propane-1,2,3-triyl 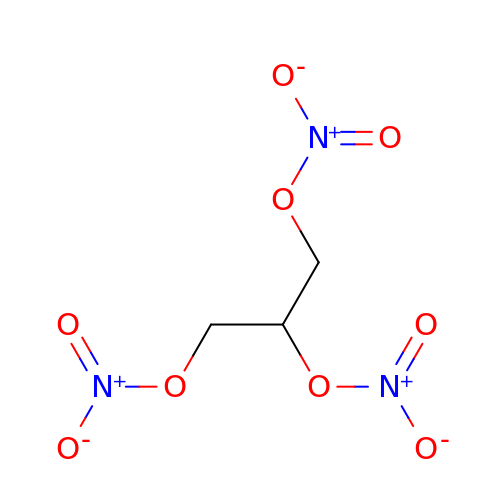trinitrate | C3 H5 N3 O9 | SNIOPGDIGTZGOP-UHFFFAOYSA-N>[2x]MKRLKKTVASLTAVALLGMGSAAVWAKDIKPRIIRFGYGLADDSPTGKASAHFAEVVSKLSDGKMKVKTFGNGALGPDEQLINSLISG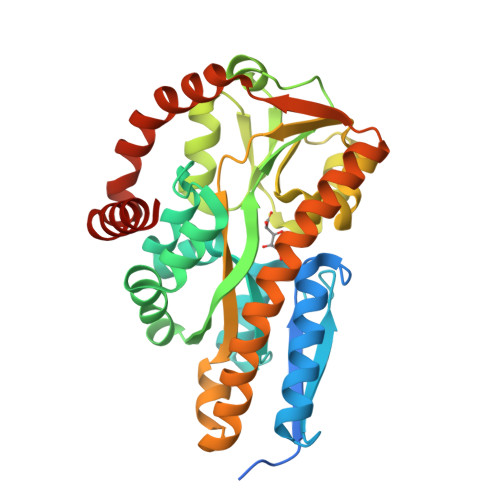SGEITFVSTAPIASLIPEFGVFDLPFLFDNEKVADTVLDGPEGKKLLDKLPAKGLIGLNYWENGFRNITNSRHEISKLDDIGGIKLRVMQNQVALSVFKGLGANAIPMPFTELFTALETKTVDGQENPLSTIQTSKFYEVQPYLTLSNHVYTPFVFLASKKWFDQLSQDEKDVITQAAADSQAFQRKASRQGNEDALKYLKEHNVKVAEFSTEEREKIREKVAPIVESLKAKIGKETVEGVLDAAKKASGA Bacteriophage Casadabanvirus JBD30, from the order Caudoviricetes, is a temperate phage that infects the bacterium Pseudomonas aeruginosa. The virion of bacteriophage JBD30 is composed of an icosahedral capsid, long flexible non-contractile tail, and a baseplate. Using its baseplate, JBD30 attaches to Pseudomonas aeruginosa via the bacterial type IV pilus, whose subsequent retraction brings the phage to the bacterial cell surface.

Reconstructions of the whole JBD30 baseplate and its parts enabled us to assemble a composite map that combines the localized reconstructions of the baseplate core, receptor binding proteins, and tail fibres. The bacteriophage JBD30 baseplate is composed of a trimer of distal tail proteins, three tail fibres—each composed of three heterodimers of gp47 and gp48 subunits, three upper baseplate proteins, a trimer of baseplate hub proteins, and three trimers of receptor binding proteins. The upper baseplate proteins together with the distal tail proteins form attachment sites for the tail fibres composed of three gp47 and gp48 heterodimers. Three tail fibres resembling bent arms protrude laterally from the baseplate. The baseplate of JBD30 is terminated by a tripod formed by three trimers of receptor binding proteins (gp54). The interior of most of the tail tube is occupied by a trimer of tape measure proteins (gp46). However, the cryo-EM density in the tail channel is not well resolved, except for the part in the baseplate core. The resolved density enabled building of the structure of the 33 C-terminal residues of the tape measure protein, which form a coiled coil. Residues Lys1149, Arg1151, and Gln1152 interact with Ser59, Asp61, Ser64, and Gln66 from domain I of the upper baseplate protein, and thus position the C-terminus of the tape measure protein in the middle of the tube. Methionines 1130 and 1134 from the C-terminal domain of the three tape measure proteins coordinate a putative ion positioned on the tail axis.

>MATNQQLSIALRIQADLAEAQNALRQLTGNLQQVDRGAVQTRSELSAMGGQLDSLRAQVLGFVGAWASLSALGGLVTMVDQYGQMADRIQMVTSSTAEYEQVQARLLETASRTYRPLAEAQELYIRTADSLKSLRYTTEQALDITDSFSFLLVTNAASADRAASAIDAYSKSIQTGKVSSDAWQSIMAAMPSLVNALAESTGKSTEEIRKLGIEGSLSLRDLNEGLRKTVAANREAADNMGTSVQDALVSLNNALSAYLGELNRTYDITGSVSSALNVLAENMEVIVKLFGVAAVAGLTRYVASLTLATQAKLAAVLAARAQAAEELRTAQAQVASTAAAAANARAQAGLTVSHTQAAAAEAAHTAATQRLAAAQLAAGAAMRGMLAVIGGPAGIAMLVAGAAASFFLFRDSAQAVKSSLDDLSEPLDQVVERMGKLSEIEQDRELTRLSEQIDGLRQTAVEAAREMREVASTALYGARLDRIPSAEAQQALQPLIDASADAARGVEVDWKSVMDTLAASGAVPDSLKRKLLDMAAGQAEAGRTATELGQRHAELKARLEGSTAAINENSDALSKGSDKAAEYIQSLRLAIADLEDPSVLGKAGRRLQQFGADLNAEQSAEILRLETLKANTEKAAQAREDARRKAESSARQQASTAEQLAKSQEGYVAGLEKQARTLGLTSAEVRAYELAEKGLTGALHARAAAALAALAADEKKRQADANARTNAGLEAEYLRATGRTVDAGLLEIRTKFDAMRRDFEKAGNDAGLAWIDKLIPVAEAKVRLDDVKQQMDDLLADQQRAESSVNVQQDAGVINEMDARQRILDIHRATYEKLQQIRPILEQMARQPGEVGRAAAESLAQLDAEAARLQQTTTLLETTLRDGLTTGFTDAIKGLASGTMDLRDAITSLGEAVLNALVNMAAQNLAQSLSSGIMGLFGGGQQDTSMTTGAAAVTASAGALSTAGASLLTGAAAIQAAAASLAAANGVQGLGAAAGGAGAAGAAAGGGSWLSSIAGIFGFASGGHIKGPGTGTSDSIPILASNDEFMTRAAVVRQPGALAFLEQFNRYGMAALAGWANPVRHATGGQIGTPAPNLPAPVRAGANLPEPSKNFSTSVANSIYLHAVQDTDQMAADMWAGKGGEHFLVWLNKNRQAVKQII[3x];>MATFPGFQVPKPVEGIVAGITPNIDALELNQDISLAAVAASTWGGAYGAHQPVEVIHSTYQAVHQSALEENYYNRLWLIPTAMELGNVVSTQIRPASVWNAYFSPRTLTAIDREAADGITLSGQASPPLGFAALEERTWTVSIGTDGPPVVNARIVWRLQGEPNLVLVITGNRIIAWTFAPDWGDSIVERLSASTNILQSESAVTQRRAMRLAPRREFDANMYAVDRERQLLDMTLFGWGARIWALPIWPDIQLLHQPLAAGSLGIPCDTAGLDFRDGGLAMLRGEDAFTYEVVEVKTVTASGLDLVRPVQAAWGTGSRLYPVRTAQLTEQPTLTRLTDTAQSARVSFLVMEPSAWPELMPATTYRGRPVLEQRPDESEDLTSSYQRLLSTLDNGSAIPRVTDVAGMALPVIGHRWIGMGRAERSAFRSLVYALRGQQKPLWVPTHADDLTLVATVSQLSTALDVRNIGYARFANGRPGRRDIRIELYDGTVYHRRILTSTELDADTERVAIDAALGRLVEPTDVARICFMALCSAASDVVEIEHVTDSEGVATAALTFKGVRDDEF[3x];>MTLYMGPNTGLLINGLPGEGHYSDLIRMWRWDDFLRQPVVKGRVATLPTTGQAEGDTYIFTGSGSNQNRLARWWATGATTAIWEYMPPRLGWRVQVANETTPSGQVKTYEYSGTAWVELVGGMSDAPSDGKAYARESGAWTELGSAAKSALNVLPFMNLMPDMGRFAGTAANPLATMFTTSWTPSSFLNGWNGATVADGGKFAFDNSTNGGAGPALNARVQALLAAMGRTWTSVSRYGVEFFTAVLTAGSQTTTGSAGADGVTRYLCCSNGSKTVFNAGGWATVVMWLRVESGSAHISSAPYTTHRLWINGAVAAPGVVLPANQWVHLRFSMQSYNGYDNACPYIYASAGAQIAFACPAWFGGLVDPGIHVAPILTINGASA[9x];>MAYFTGTANNPADLLAKVRVHAESLGWVTDRASASEWLCHNADGYWSFNAGANQFQMAGNTGFDNSLAWNAQPGNSVQNNPYSSKGPTVAQLSGGPFTRYHLFATAAYLHLHVEIAAGQFRPVMIGSLNKRGVGYTGGQYVCGSFIYTPGQALTNNWSSHPFDGYHIQYSNSSCMLRLDGLDGGPSPEWLPFDYTTNVPRRVVGPGRGNYSSQYHPDVGLIDASANELNSSTTTVPCAIYAFGAQQRSRYVGEVPDFGICNMAFLAPGDPLVVGSDTWRVYPLLQRGTATDFDSTSAWVGYCFRVVE[9x];>MATEFGTAVNHADLVERLVQFLTASPDLVAAGQAYEKVFDNTIPASGTAIAVRQVTLRAPGLGGTDAIYMGIQSYGDTALDYYNLRLMGGTAFNPGAIPPGGDYWTAFANYSPRVQLLAWNQPMPYWFFANGRRFWIVVKVSTIYESAGAGFILPPCPPSQYPYPLAVVGSYRGDVATRWSDVSDRHRGISSPYERSCYLRDPAGRWLGFTVDGGAANESDYNNRTLLPLGCGRYAGSSDTVVKQLRDSFGKFPLKALQFVTRETEGRRYLGDFDGAFYVPTLNSGAEDVIVEDGVDHVVFQTAWRSGNPWLYAIRKD[9x];>[3x]MSFNSRESSLADGQPVRLYQFSRGAIRWSYNSSDRDITYQNQIFRTVPGGITDNGIICSGDPQSDQFVITAPADLDVALLYKTRSPSDAIDLVVYDMHYGDAEAAVSWVGQIGDVDWPTVDSCRITCVSEDELMDQPGLTDTYCRTCTAIVGDHRCKVNLVPYRVTLTPQSVSAWVISSGVVAGYADGWFTGGYVEWQVDGDNYDRRFIEQHAGADLHILGGTEGIPAGGQLRVYPGCDGLAQTCDDKFSNLPNFRGFNAMQGKSPFDGDQVW;>MGAKPKAQTVGWRYYFDIHFALGKKVDEVCAIRASGKTAWKGSITSNGQVRINAPELFGGDKGEGGLDGTLDVLFGEEDQGVLPRLAAMLGGLVPAFRGVTTCFYSGLVTSVNPYPKKWEILRRGGNRLWDGNPWYPEKQFVWLADGQIKAMNPAHILYLVYTGRDFRGLARTRMDEASWRAAADTLYAEGFGLCFEWTRSDSFKNFCETVKSHIGAEVYPNRQTGQISIRLLRDDYNVADLPLFDEDSGLLEITQEKTGSTSLAPSQLIVKYIDQIDGAQRQIIVNNNAVAASQGRRSSEEIEFLGVPTGELAGRVGEREMRLKTTGLKRYKGVFDRRARSLNPGQPFLIRSTPRGIPETVVRVGRIEDNFLGDGKITLTVVQDQFNLPATTGVAPPPPGWTPPDRTPRAITVRRLIEAPYRELAGVIDPANLQLLDVSASYLAALAEAPTSLSQSYTLTDRVGSSGAFVDRGTGDWCPTGLLAAELPLAAGPNVVTLTNATRLEDVTVGQAAVVDDEIVRVDAVNYASGTVTLARGCADTVPAKHLAGARVWFYDTFEAVDETVYSQGVTLQARLLTNTSEGQLAPALAATDSLTLTGRQGKPYPPGQFRINGSAYPTKVYGALSVSWAKRDRIGQADQLIDTTVGNIGPEDGATVTLQVYSGTTLKRTYAGLTSSSWSYPLAEDMADGPLQDVRLVLRSVRDGIDSWQQHDITIERHGLGFRLGEELGGVSA[3x];>[6x]MAQETYFYGQGEIDAAPIVNGVLGKWRWIQDVSAMSIQLAVEKVEHKESYSGQKALVRSFPIGKTATVNITLHSIGPDNLALTLYGKVVAKAAGSVTGEVLPADLVAGDVIRLANFGVSELVITDSASSPAPLDPQYYALRADGAYGEVQLLGLPTPAPTQPFKAAYEYAATKQVGMFTAPQPTVALRYKGINLAEGGAPVIVELYKVATDPLQELALISDGNTVAGMQISGGILLDTSKPDTGDLGRFGRIIQLG> MDTQTHLNFTQIKTVDELNQALVEAKGKPVMLDLYADWCVACKEFEKYTFSDPQVQKALADTVLLKANVTANDAQDVALLKHLNVLGLPTILFFDGQGQEHPQARVTGFMDAETFSAHLRDRQPGLVPRGSG

The transmembrane thiol:disulfide oxidoreductase DsbD is a three-domain protein responsible for shuttling electrons from the cytoplasm to the oxidizing periplasm of Gram-negative bacteria. Its central domain (tmDsbD) is located in the inner bacterial membrane and is flanked by two periplasmic globular domains (nDsbD, the N-terminal domain, and cDsbD, the C-terminal domain). cDsbD, like many proteins involved in periplasmic oxidative protein folding, adopts the more conventional Trx fold. Its role is very specific, to acquire reductant from tmDsbD and transfer it to nDsbD.

We chose to study the Q488K variant of isolated cDsbD and full-length DsbD because of the key role of Lys-57 in E. coli thioredoxin. Despite the presence of reducing agent (TCEP) in the mother liquor, both proteins were found to be oxidized with a Cys-461–Cys-464 disulfide bond clearly present. Cys-461, Cys-464, Asp-455, and Glu-468 of Q488K-cDsbD overlay well with the same residues of wild-type cDsbD. However, unlike E. coli thioredoxin where Lys-57 forms a salt bridge with Asp-26 (equivalent to Asp-455 in cDsbD), Lys-488 is in close proximity to Glu-468, and the two residues have hydrogen bond interactions with a bridging water molecule. The Nz of Lys-488 has a high solvent accessibility (36%), which makes it possible to interact with the solvent-accessible Glu-468 (side chain solvent accessibility 36%). Asp-455, which in the wild-type domain forms a hydrogen bond to the side chain of Gln-488, is just hydrated in Q488K-cDsbD but still remains almost completely buried (side chain solvent accessibility 6%) leading to an elevated pKa of 7.5. The Nz of Lys-488 is more than 11 Å away from the thiol group of Cys-461; therefore, this positive charge does not affect the pKa value of Cys-461. The closer proximity of Lys-488 to Asp-455 ensures that this residue has a lower pKa value (7.5) than observed for Cys-461 (10.5). A pKa value of 10.5 ± 0.2 was observed for Cys-461 in Q488K-cDsbDred (closed circles); this is very close to the wild-type value of 10.6 ± 0.2. Therefore, we can conclude that Q488K-cDsbD has similar biophysical properties to the wild-type domain, and Q488K-DsbD functions equally effectively as wild-type DsbD in vivo.>[2x]MEKSNPNSTSKPHVFLLASPGMGHLIPFLELSKRLVTLNTLQVTLF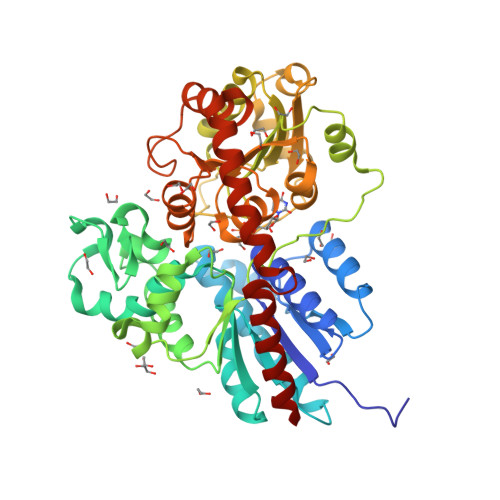IVSNEATKARSHLMESSNNFHPDLELVDLTPANLSELLSTDATVFKRIFLITQAAIKDLESRISSMSTPPAALIVDVFSMDAFPVADRFGIKKYVFVTLNAWFLALTTYVRTLDREIEGEYVDLPEPIAIPGCKPLRPEDVFDPMLSRSSDGYRPYLGMSERLTKADGLLLNTWEALEPVSLKALRENEKLNQIMTPPLYPVGPVARTTVQEVVGNECLDWLSKQPTESVLYVALGSGGIISYKQMTELAWGLEMSRQRFIWVVRLPTMEKDGACRFFSDVNVKGPLEYLPEGFLDRNKELGMVLPNWGPQDAILAHPSTGGFLSHCGWNSSLESIVNGVPVIAWPLYAEQKMNATLLTEELGVAVRPEVLPTKAVVSRDEIEKMVRRVIESKEGKMKRNRARSVQSDALKAIEKGGSSYNTLIEVAKEFEKNHKVL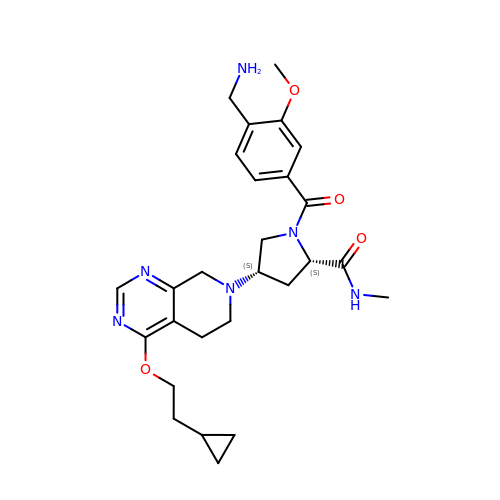(2~{S},4~{S})-1-[4-(aminomethyl)-3-methoxy-phenyl]carbonyl-4-[4-(2-cyclopropylethoxy)-6,8-dihydro-5~{H}-pyrido[3,4-d]pyrimidin-7-yl]-~{N}-methyl-pyrrolidine-2-carboxamide | C27 H36 N6 O4 | PZBPHXPZLFDRAP-REWPJTCUSA-N> ASKSEKNADAPKTFSYVYAVDPSSLDYSLTSKSSTSDVIGNVVDGLLENDKYGNLIPSLAEDWSVSKDGLT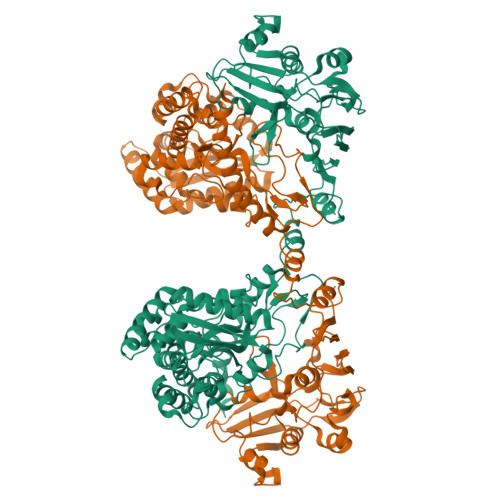YTYKLRKGVKWYTSEGEEYAEVKAQDFVTGLKHAADGKSDGLSLVEKSIKGLEAYVSGETNDFSTVGVKALDDYTVEYTLNNPESFWNSKVTTATMLPVNEEFLNATGKDYGAPTPSSILYNGPYFLKSLISKSVIEYEKNPNYWDKENVKIDNVKLTFYDGSDQESLIRSFTQGAYTTARLFPASSNFESTKKEYGDKIVYSPQEATSYYLTVNVNRQSYNKTAKTDESQKTSTKEALLNKNFRQALNFAFNRHAYTAQLNGEEGADKIIRNSLVPDNYVQVAGKTFGQLAQDELLKYGEQWKDVTLTDGKDTIYNPTKAKSAFEKAKSELQAKGVSFPIHLDVPVEQTDVVAVQQTNSLKQSIEETLGTENVIIDVLQMTDNEKESITSQAKVPTQKDYDLNGTGWGPDYQDPATYLNILDAKKGSALKHLGITKGKDPEVVAKVGLDEYKKLLDDAASETSNLDKRYEKYAKAQAWVTDSSLLIPVASSGGSPMVSRTVPFTKAYSQVGIKGDPFIFKGMELQNDIVTTKEYDAAFKKWQKEKLESNAQYQKDLEKHIK> IIDGAPCARGSHPWQVALLSGNQLHCGGVLVNERWVLTAAHCKMNEYTVHLGSDTLGDRRAQRIKASKSFRH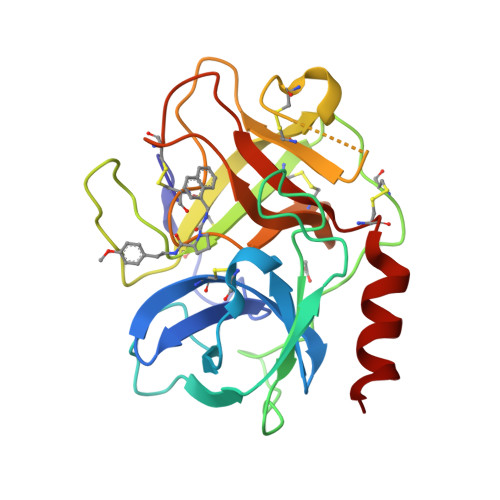PGYSTQTHVNDLMLVKLNSQARLSSMVKKVRLPSRCEPPGTTCTVSGWGTTTSPDVTFPSDLMCVDVKLISPQDCTKVRKDLLENSMLCAGIPDSKKNACNGDSGGPLVCRGTLQGLVSWGTFPCGQPNDPGVYTQVCKFTKWINDTMKKHR>[2x]ETGELKIECPHTIGLGQGLVIGSVELPPVPLTQVESLKLESSCNFDLHTSTSSQQPFTKWTWEMKSDLAENTQASSTSFQTKSSEINLRGLCLVPPLVIETAARTRKTIACFDLSCNQTACQPTVFLIGPIQTCITTKSCLLGLGDQRIQVNYEKTYCVSGQLVEGVCFNPVHTMALSQPSHTYDIVTVMVRCFLIAKKVSTGDSMKLEKSFETLVQKTSCTGNGFQGYYICLVGSSSEPLYIPTLDDYRSAEVLSRMAFAPHGEDHDVEKNAISAMRIIGKVTGKAPSTESSDTIQGVAFSGNPLYTSTGVLTAKDDPVYIWAPGIIMEGNHSVCDKKTLPLTWTGFIPLPGEIEKTGTKHHHHHH

Hantaviruses, a geographically diverse group of zoonotic pathogens, initiate cell infection through the concerted action of Gn and Gc viral surface glycoproteins. The ∼1,150-amino-acid glycoprotein precursor is encoded by the M segment (Schmaljohn et al., 1987) and is co-translationally cleaved by the cellular signal peptidase complex at the conserved “WAASA” sequence (Löber et al., 2001) into two structural glycoprotein components, Gn (∼70 kDa) and Gc (∼55 kDa). Low resolution three-dimensional (3D) structures of Tula (TULV) and Hantaan virus spike complexes, derived by electron cryomicroscopy studies and combined with biochemical analysis, revealed that Gn and Gc form square-shaped oligomeric complexes on the virion envelope (Battisti et al., 2011, Hepojoki et al., 2010, Huiskonen et al., 2010). Here, we describe the high-resolution crystal structure of the antigenic ectodomain of Gn from Puumala hantavirus (PUUV), a causative agent of hemorrhagic fever with renal syndrome.

To facilitate soluble protein expression, a PUUV Gn construct (residues 29−383) was truncated by ∼120 residues prior to the C-terminal transmembrane helix and transiently expressed in HEK293S cells. The crystal structure of PUUV Gn was determined to 2.3 Å resolution using the single-wavelength anomalous diffraction (SAD) method. PUUV Gn forms an α/β fold (∼40 kDa), consisting of five α helices, a 310 helix, and twenty-two β strands. The β strands assemble to form five β sheets, which associate together by the formation of a β sandwich. The two molecules of PUUV Gn present in the crystal asymmetric unit are almost identical, with differences being limited to solvent-accessible loops (0.7 Å root mean square deviation in equivalent Cα positions over 327 residues). For both molecules in the asymmetric unit, three loops (residues 92−102, 204−208, and 292−300) were not clearly visible in the electron density, and it is likely that these residues are either naturally flexible or require an associated protein, such as neighboring Gn/Gc protomers, to impose order. No higher order oligomerization was detected from the crystallographic packing, supporting the hypothesis that the Gc glycoprotein and/or C-terminal regions of the Gn may, in part, be required for tetramer formation (Hepojoki et al., 2010). The PUUV Gn fold is stabilized by seven intra-domain disulfide bonds, a pattern well-conserved among hantaviruses. The PUUV Gn sequence exhibits N-linked glycosylation sequons at Asn142, Asn357, and Asn409 (which was not included in the crystallized construct). Electron density was observed at both Asn142 and Asn357, with the glycans extending away from the protein surface.>MASNFKKANMASSSQRKRMSPKPELTEEQKQEIR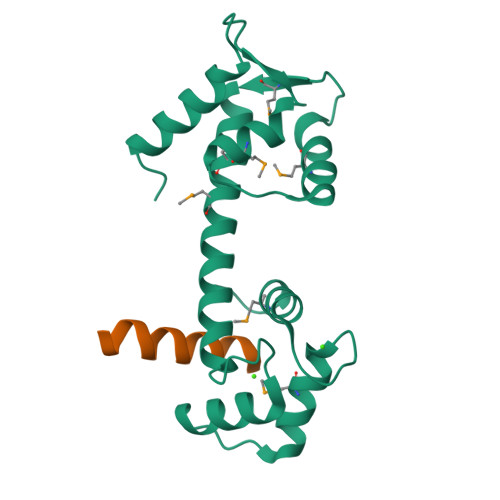EAFDLFDADGTGTIDVKELKVAMRALGFEPKKEEIKKMISEIDKEGTGKMNFGDFLTVMTQKMSEKDTKEEILKAFKLFDDDETGKISFKNLKRVAKELGENLTDEELQEMIDEADRDGDGEVSEQEFLRIMKKTSLY[2x];>[2x]NWKLLAKGLLIRERLKR> MNPSQTQKGKIQIQVSRGSIDLLVRTMYEDINNIKLKNERFQKKKRAEDERRRRERYAEIQQEAIASGKKNAALEMKWAELKELDECEELNREMQDQQQTFQQIIEGKENLRKEFEEELKRKDDEYVKMLKEQSNDIKDMISKMRSQFYKIRDANMQELEDIERHFEQERSNLLNEFKAKIQATFKKHLDLEEQYVKEHAKTEEEQTKNIEDLRIKGAKHYAELKITMETEIQDLEKCFEDMKALYQLITEKLDYSLKVLQEKFHENNSMCDELKRKENNFKNRLKQLTKDYKQYDKKFKLENKNLTQEYKRIIRQFKELQKKFKHFEKADLDKYSEIQKMNEAEVKELKDKIIKCNITIHIQQLGMQWIPPQSEEEILAQQKLQLEQGGKAEEEEEREFEFCISEIKIGEICNIILEEADFLIDDKLREELEGSAEPEQIFQRLDCIKKCLYIDSEDEMNLFFRELITKCRVKSAEEIEEEARKQLLLLGLIKEAEENENPEGEEVQQQEGAQQKKKEEGNKKDDPKGKEGAKDSKENANPQGQNKSNQDERKKKKDGQDDHAGQGQGQYDSNQGGMGENQEEGENAEGQENLEGEIEKEIDLENTQINLNEVVKFLQNWQANKDKRKEKLEKESSKKAVKQETEREKKERIAREGKKYWEKLTQVLPERTFRIWNVNFFKFSFEKQILLNQINKLRFWTDLCPNIMNFFWTDKNQSKKPVNCITKMKNQRIFQINTYKLIMNLLSALQDSLIQIKDKDDFIQTKISTNLFTFHNFQILLQIFIVNQSFLFIRLCQSYSKKIILLIKNINQKLFNLSNFKNQFSF;> MALLGKTLKGRSTRPGGIPQKRNIKWRQLAKNQEEFDQLKQLAKMKREGLKARIKDEQKVVTFNKKKLITYWRKIMRIAKTEQLKNEIDIYSQNNQRELDSKEAFIQMLDKNLDEAEDQFQIALRNHLIHIENLMQLQEARMRGLAEEFNRDVNILETEFDLEREEMVKTHKTQLKELEDMIETVKEEDKKKTEEAQNEFSQFKEETKNKNLEETNVMKIILETKQTKYYTELEQMNSKFQSDTSNKVKDHQFYHAHNKNRKQEIDRYLRTISSKKAKIDLMKLKILQHCKEFNARNSALKKEKENISRNYHELKLKMQKFREEESRRLKELSNNSRNAVLKLREYCALGEKILKTAELCRRLETEKEKVLPFYESSVDEDQIPEQLKNEFEHLKKEDAEEYAYLNNFYKRYNKVLLDKLAIEKQKENLQRDNQLLKSLLKQYLDGISLNDDVLKNENNPLLVVNHKFNLGKMPVEKIENKTVIEGVFEVRNTSHQLQGQRAPPFQ;> MSNYISNYVQSTIVTKTVQNKDKKTGKNSVDPRVINEQLILDAVKQFNQENNKITTENIILQQLRQLQLSFKNILKIQHLQGLERLEKLQLDNNIIEKIENIDHLVNLKWLDLSFNCIKKIEGLDKLKELTDLSLFNNYIEKIEGLHNNTKLNVFSIGNNRLKSYEEITLYFGYKPRGEEGTNDRPEFKRLQVLNVSGNPFTKDKENEYKNHIICAIPNLKYLDYVFIDEGDRQLIRQDEQISNSYNFTTTDYYQQMQAQEQKEEMDRQTLKKKKDARMDILDNLKDEYLKIEDLQRVKIIKPNQINEEIEKYCGKINDHVVEMQAAVIQKHQLILQEMSKTEVSYKEQEALHEKETLQILKEFEHEKKVEFRNWEKEAANGDAKKEESRLKTLLQKTTSLKNKLMDIEIQLVEELEAIFTDYDTKKKETAWKDIEEIIVLGQKKIEEENVKFYSNLNVIKNKEEANYNSTQQQQLEEENNEEDDEKASLLENKEQLAQMIGNIKETLIDSHTKIILSAQMELQKDLAEYAKQQKNKMYERNRKNISQIIAQIDAYQTEINEKLKQGDDESDHEN;> MSKAAKAKKNVPVVSKLEADARKAAEGVNDNESEEFKKAMRKEARALVEQFNEEKKLLAFYQQERQKINYNWIIAKKELEDKKSELINKEREIQDLQENHFMTLNVYKQKIKHLLFQNQDQQSELKKDVEVTLKQLEDQHRIKSRELKTDVRSLKVTKKEQEISQQDYLFALKSEHDKQMTLMRQ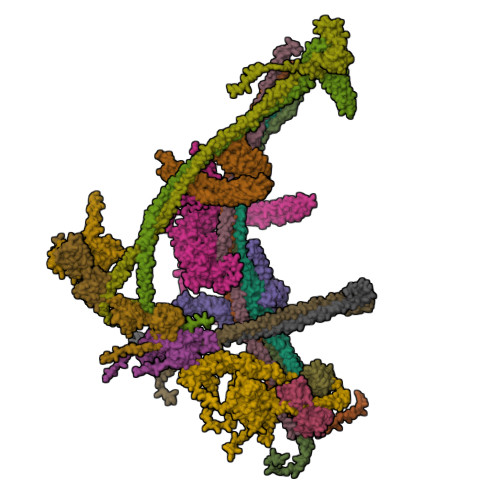DYERQVNDIKRKYDLKMQNLTKEMEEARAAMIKQLEDNKNQKIAEIIKEHTQKYNDIKNYYSEITATNLDYRKTLKNEIKELQTKDEEYKKTLQQTEKGYKELNEPLQALGIEIIQLKKQDEEQEAIIKEKEELKQKIDNQERLFRKLEYEYEVKLQQFQYLERERNALYAKFNQTVFEIHQKSGLENLILEKKVTNLREDLEIKDLQIHQVLTAANIDPNSVGSINKSLEEVESLKNELISELQAQLKQIRKAHSHMVKAYEGKLSEFVIPVEELGFDPLVPTNTD;> MPPKKAKGKKKKEEEPDDEYKSMTGADLTQTLEKLKERVNEMRTNRNYIQMDRDMVENFYHNTLKEISEVKTKISNKETEAEEKESKHRIDVKVFLQKVKHLEYEQEKSNLNIEDDGKKAKEKEDAYFEDITKNMKQLKTQLKSEYLEKEKANIQQVQEEKKDHQSLLKIQQKKFDELINNLIIKYEERLAKLKEDLELKLKVEIHELEERKNLHINELMNNHEKAFAELKKYYNDITAENLNLIKAHKEKIAQIYANIQLNTKNVADNQAKNEQLKEPLAKHREIRNKLKEDLKQFAKHKMSLQNLKSKAITLKDKITKLERDGKDLDEKYEKVVREKQELEKKFEDITQEVKKNADLNNNVLSNRLQILLKEYNNKEEELRTIIDNAGLDHNLHEQLKQRVQQSIEAKNTLIKNLKYSIHHATKAYNDAIRVYEAKLVEFGIPIEELGFQPLETITSSMPAGLVSS;> MLAKKLALARSQGKPDPFKKDEFPLLQHIAVEVVSQNYILYPDLKGVPENVRDTIISKITTDLDILTMAPNIDQESFWQRACKNRWEKSQKSINIEEHGRSWKVAYLERYMEEFLTNIQNADDPNKKQILQAELKAAASWIHTLNLQNINQNIDIDFICKYLPLLTSLTLTYGTKYSGMDYNKQSVGMKLSEAANLGEAIKNCYSLLSLNISANMIDDDLLRFIMAGVNMNISLIELNLSHNKIEDQGARRIAKFLMRNEILLYLNLGNNLIGYEGSRYLAQALKVNKNLQSLNLKLNNLGDKAGKKLFQDLMLNKTLLELDVSGNQFEFETALKLSDYVADSMCGLKVLNIANNDFNDSCYENLKTGFTKNYSLAKLDLRGNKFSKTQEEKEQELKDPFRMFNLSQTEKELTQIIIRHDLTAQKIQFFSESDLDKIKQLKELQGAKQEPEKVIQQDQNKE;> MGDKKGKKKGGGEEDESTLQLSRQYKKKCELNGINPSKLFKEKLDFAVEEDENIEKIHLWEELGPVGVRSIMDSLTEIPYLHTKSIRLWKVKAQDEGTRTICNYMEKSKTIEYLDLMDNQVGSLGCEFLGRVLHPQIEIPLLKLKLDHNEFGTEGLMQLAAGLCMNSVLEKLSLNYCAITAEGSKYIQQILSFVNTNLKKLKMKGNLLKNEGVHQLFRAFKVNKTLEKVDLSDNQFDTTLGDDQDPEANPNFFETNKDAIEHNKQIIENICEVLKAADTLLYYDFRFNNISKTDAKAIIDCLEANKNIYYMELSEHIPKDLIERKKGLMKKRKPKKKKKKKAKKK;> MDHNEGGYSHHQIEGQEGQQQQAPVGGGGEDIFQVLENITQVQNEKLKRCQEFKEQENIPRQYIENSPKEELVLEHVIQFKRQFQYQLYYEDKRDLFLYPKNECDVYKFICTTIRPTKLGFLELYDYQQCSKYLSEFVQYEELDPPNEFPLVIPSPTNVAVWQKGDCFDMSILLCSLLIGVGYDAYCVYGKAPREITTRNESLMECLFLEKGKYIEENDKKPKQTLEQNENALLKKPIAHSKWDQTQETKAREAEEEKRRIALTINDDEPDELLEDPYQGQRVHCWVLLRSGKRDVQQNIFIEPSTGRMYSPSTCPYECVDAVFNNLNFWINMKPECEVKNLNFEEMDSSLNWEYVMLDTLLFNKGNGNDEEGNENIDDPLNKQAQRDPEQEQLQDIAQLLDMPPPWPPKIYIDKEKFLMGTPLGEGTVYYNKVKVDNYAPYSQPDGLVQKITIFQDYKRLKVKEYRYFYKHRSDKLSIRRRYPFEFKTIEEYEPQKYENKTIPQALQQWRQVIQIDRHLRIIKYYHNRNHDGLIERVEQIGEKTMMFYQNRDDRVIYRSIRFDNKRAPSSQNNDKVFQDNHVGDVQITKMTQKFEKNPHYPANEQIQKMVIDLIKDKVIVYYHMNDGEITPIVKIYPRDSMHGFAKLNEPGGDNKIDDPLVQLENTKMVNLEKDCLNQLKQQEKIARDDEKTIREGEIRLEKTLYDKARDRFKESSKKNDDDLAKDAAASDYLYPYLEKRKLLGVSEINAQVAMEIKNEVMQKLKERLLSRAEIIQRRLEEQRQVLEQKEAQVAKRQEIDPKQEEEIRDINFKIDILEQRALRFESMALQKYEEMDNRLNKDARLAALHRK;>[2x]MYDPNTSQTEKQKQEEFLKLKIQEAFNLFVKDKKGIVDKREIPYIMRYLGQFPSEAQVRDAILPEIEEDEPSEFIKYSKFEPYMLKVLKEREYEPDDPEALLAAFKLLDQEGKGYIEIDMMKTFLEKQGIEFREQETKSFIEFATNKDPNATVIYYEDYISRLQAFTDKHIESVMKGYNNFQVKK;> MNQIDAHKLTIILRDATERLTFLDTINRQDDLSSELAGYEISKLLKKQKNLENQYADLVQLRTSLTGIQNKKNLIETQTKIVDVAQNLKESTKKLCRLFKENPDLESDALKVKKDRIQFMAVIEQLIQMVQNNSLTKFQSMTTLELEDQDRLRKLIFREKELYQEIKKLQFDRNQENKEYDNEQKDTNLKIQNLKERLLYKKARAQLKNQYKEKEARAEEGTQQRMYEFEQKQLKEKINNLKQKTDTENMVHEQLRNFLIEKEDQIKQKSDEWAKKVETCREQLQEEIDRLTVEKEKKQEELRELRERDQKEQEEKDRRERQELEEADRKQQEELDQIRLDNAIKLIQIEYQEWKDAGGGKKKRKKGKKKKK;> MQNLSKMQSRLHPRPEGEGGGGGGRTKEKGKSLQETHKEMLKNIESTNIGKPTIVEAQRILKIIDNLSTNLTIFIYLDSELISKFLDVAKHSKLSKDLVSKLSQRCLDLLKSQAEIEAKFKPYASLLDQSNKEAEDVEEEKMIDAERLRMQLENNFKDLVRHLRNSPEDFEIIKSMKTNVNPDLNDLVHCIHCQKVIMLKKLSTASEEDENHKAQLRDLEEKIEELEKKKNKIQEDLTKLKEHRQKFSKEKKEELEKLKNEIAEVKAEKEKKASQLKNELDNRLKQLERDHLAKKDKLDKELQKLEDDFAKLKQDHANDETKLKTNKRQQQNSLADNIESYDALMKDQHQKKQEIEEELAKIIEEVDTLKQLFKEIDEEKQRERELEEEFRLKKEQWEIQERRKKEAARCILHFLMARKEKSKKKKKKKGKKKK;> MSNMMYNMKWQEAINDLMEQVTLEYLPLEQNEQQLGMKYKRDSSEWFHFWATLYIKYIDIYKKLEDCYDQLVHPQKRVLLKEMLENVIVRLCETKSQVVKYNTQYDATYKSDYPNLDELVMDLKLTPDCLDIPIPRYFREEDKKRLDERNQILDALLLEYTDTKEPQEEQYEDQNTLQADMDTAIRIIQRYERGRQGIERANLAKILKKEEEKKLERQKKLAEGTEIGEETEKDDAALVIKKYWRGYKSRKLVQDIREEELLFLGMKKVVEDPTLPESQYKQAQNKRQKMKYIQEEHEQEFNDEIENLKRLVKGNEGPDILDKMRAERREWIMRELEKNEFKEAPQDPSEFYNQQVMDPEQQAAEAAKAAEEAKKKGAAKKDDKKKKGKPSELDEFLENNKPTGPSPIVLKLQEQIEKHSGEWSKRDETNNFEQKHETELAKMLIKPVVEEQIKQQVDEMIAEELDIVRLRYDIKKKKQKKPPRPRNKGKNKKKFPGDSSNKGRDPKDILAGLVEKRVAKKLIPASLMDLKGEQNVLGKIQEIQADENLKKTEALTDAKLKKAQLEEPSTKMPDPSIAQIRQIIAEYIAFPLGSKYAKEKLDKMNYFFFMGPRGSGKTLAVRALAHECNAIVLDISPSNIDGQYTDKKQIDGMINSAFKVAKEFQPAIIYCEDFEYIFGQAKKKKSQVNPLFAKMKKPLMDFKKGKFFEPEDRVVFIGSTNRPWDCSQKEIKSFFDKKIYFPFPNYGTRMLLFKTFLEQKKVPLPDNFPINTIAHITEGWSAGSFKMAIDRVFTERRLQKINEEQIKLSEFIGPLSNVPFTSKEEFKEFKKFNQVVTGLQANYEAKKAPADDQKGDKNKKKK;> MASEDGEMPSQFEGIDPEQLTESQMQQYMMEMQRQGLLDSNMEGGQYEEGYEEGQEGEGYGEEYGDQDYDGNQNEYDSQQDSQQQGHDQVNEMHQDRYDRRVNSEISGNYEADDETLRKIRRDLLDNINLERRHRDLQPVYIDLTTNNISQYYSEYLVNNEHNQDFYENAKVRYNNLGECELCHITAKFEPDADITKEYIYDYFMEIGYLFLESEEEKRIILNPANNHIGIGVFFDEIQIVVVLILSEKVLCIQKISQPEQNKIEIRGKMLDENFGIYAIRIMNVDDQKKDIKGVGPEFIEYTRSTQEWMASFELELYNQDRMAIEYYTRVSPDSIPYKKKQSKNEKLTYKHLQLRLRTPFQIYPDPKYAAEDEKERIRKEQEILAHEEQERKEREENDAKRLKQSRKDYGDGQYDDDEHGQDDFNSQSDISDKDKHHDSMHAEQEQNQQAAQQQQDTISNKEIRQELEMAITEAQRQHDEFMLQNHKLQEEIKLLKNKNDGFVDRSNETAMNEHKYLNTLAHVHQIRLDLKQTQTRYNQMSQELQKKLEQKQKKCNEIKYAFLELKREVAKKAANSRTDKPIPEQQINEWEKAELQKSKELQELRLQILRLRNAYVKNQKILKKKEELAEGLHLIDFEQLKIENQTLNEKIEERNEELHKLKKKNTTTIQILTHTREKLGFVQGENGELNSQNVRKDQELDDMRKQLTQQKKTKDKLRSVNLTLKQQTGIVNSEELGQDYRDLRTRVSKLEEEKKRLEQKLRSMHEAIKTANQISTQNMQSQNNSLKKPYQPY;>[2x]MDNTGKLEKQLVTLNDGLPKKPAKEIIEELKHHLYQDFQKFFSEEKKQQYQNNFALFDRDNDKYINLSELKELLTSVNITFPDDELEELYNEFCLTSPEADGINEDAVFIIVSKKIRDNDKDEQLTQAFKLVEKAVNDELAKTPNETKEQEGYIRVEQFKELLMTLGNRWSEEQANEFLKDINPKSDERINYLDVVKKLMKR;>MSKKSGKGKGKNDGDELGAEKEQVLRTKVESLIQRLGHEQERADRAKAAENELRARLFDLDKDFKNEKDRLFSITSDMTRQYKQMQDELLNQVNDLNKTVIEKDEEIKKKDQQIQDMTKDYEYKLKKKDDEIQDLKRKIEEMSAEFAKMLKDTLDKMQERIEMVQWDSDTDPQMMKRLKDMTGLSNN[2x]> MSLSTRIAPHLPYLRRFARSVTGSQSSGDAYVSAMLEALVADISIFPRASCDRIGTYWLFCHLFDQTTPNIPEPLPQFGLEQKTSAKLSYLTPRARQAFLLIAVEGFNEQEASEIMNLDARDFRKLLNQASIDISQQIATQVMII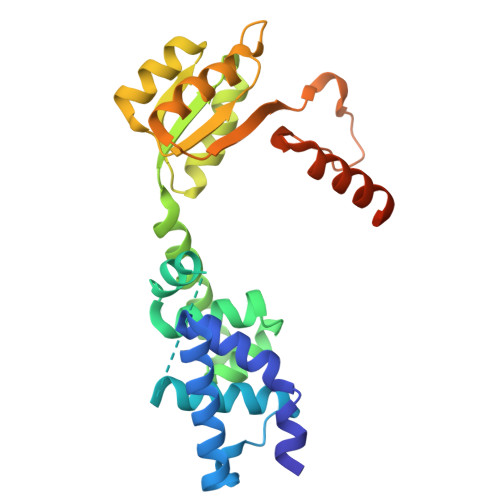EDEPLIAMDIEQMVESLGHQVVGIARTRKEAVVMYHQKKPRLILADIQLADNSSGIDAVNDILQNDRIPVIFITAFPERLLTGERPEPTFLVTKPFNPDMVKALISQALFFKENASKAALEAGWSHPQFEK>SMKLQQLRYIWEVAHHDLNVSATAQSLYTSQPGISKQIRLLEDELGVEVFARSGKHLTRVTPAGERIIHTAGEILRKVESIKQIAQEF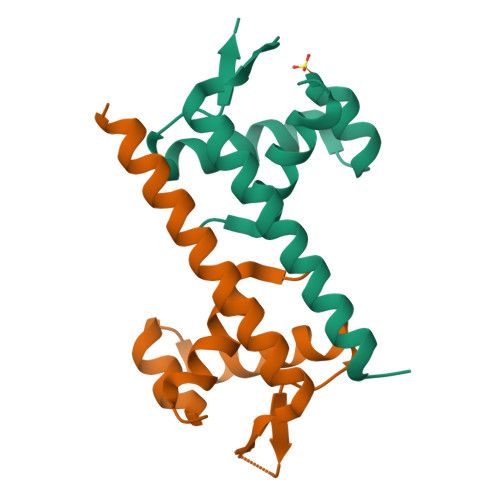SNE[3x]>[2x]GAHMGYQNRTLRSITSPLVAHRLKPIRQKTKKAVVSILDSEEVCVELV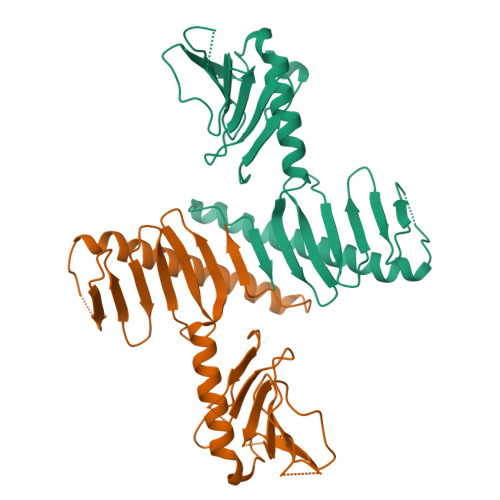KEYASQEYVKEVLQISSDGNTITIYYPNGGRGFPLADRPPSPTDNISRYSFDNLPEKYWRKYQYASRFVQLVREKEPKIEYFDRYAKCILMENSPGADFEVWFYDGVKIHKTEDFIQVIEKTGKSYTLKSESEVNSLKEEIKMYMDHANEGHRICLALESIISEEERKTRSAPFFPIIIGRKPGVDSDADEEVELILGDTDSSDNSDLEDDIILSLNE> MMKRTILQRCIQNKSLEIARISRSDINSRAHLPFNFDVCYELGSREFTLFSSVGSTSVLV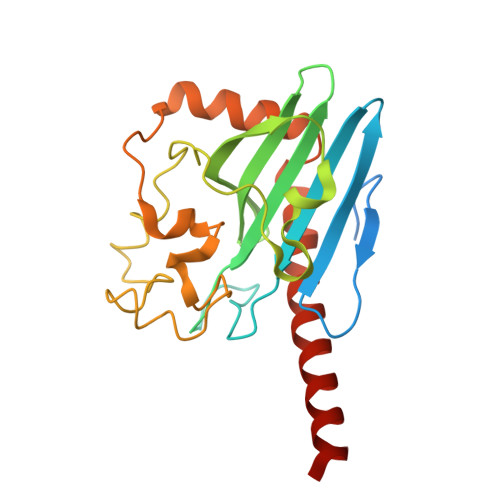FCNVSSRRLRSVKGGQGETEFPPKRLNVKRRRQSGSADRSPVVFSAFVSMPTSGLTIEALCCSSLGLLVVDGVSFHQGPLTESMIPQDAHPGPEGHYQGPLLNQRSLAEMVVNTRGCITSVDPFRQQESFFDGHVNPWNARSLRFGHVPVHTAKPGFSDALCHFLEVFGVNDELAFFVEDFAHLVHREEETAWTNVLKTMMGGR The periplasmic binding protein (PBP) CeuE1 is an important component of the Fe(III) uptake system in Campylobacter jejuni, a commensal Gram-negative bacterium in the avian gut, but a common source of food poisoning in humans. CeuE, an integral part of the CeuBCDE ABC transporter of C. jejuni, is responsible for capturing Fe(III)-siderophore complexes in the periplasm for delivery to their respective inner membrane transporter. C. jejuni does not itself synthesize siderophores, but capitalizes on their secretion by other bacteria, such as E. coli. Here we report a combined solution and structural study of a series of synthetic tetradentate analogues of the enterobactin-derived bis(2, 3-dihydroxybenzoyl-L-Ser), to explore the ligand-binding promiscuity of CeuE, both wild type and with mutations of the Fe(III) binding residues H227 and Y288.

Fe(III) complexes of 5-LICAM4−, 6-LICAM4− and 8-LICAM4− were co-crystallized with CeuE and their crystal structures determined. The structural differences can be quantified by calculating the mean planes defined by the six carbon atoms of the two catecholate rings, and measuring their inter-planar angle which is 97°, 111°, 110° and 110° in CFe-4-Lic, CFe-5-Lic, CFe-6-Lic and CFe-8-Lic, respectively. In contrast, the longer and more flexible linkers in Fe-5-Lic, Fe-6-Lic and Fe-8-Lic can adapt to both the geometric requirements of the Fe(III) center and the binding pocket of CeuE. The Kd values of Fe-4-Lic and Fe-6-Lic are similar and lie within three standard deviations of one another. This indicates that the entropic cost incurred upon binding of the ligand with the more flexible 6-atom linker is compensated by its ability to accommodate the preferred octahedral coordination geometry of Fe(III). In addition, the affinities of CeuE for Fe-4-Lic, Fe-5-Lic, Fe-6-Lic and Fe-8-Lic were determined using fluorescence quenching, which yielded dissociation constants of 21 ± 6 nM, < 10 nM, 33 ± 8 nM and 58 ± 8 nM, respectively. The crystal structures of all three complexes show that the siderophore analogues are bound in the Λ-configuration, as previously reported for CFe-4-Lic20, (CeuE)2-[(Fe(MECAM))2]6− 19, FeuA-[Fe(MECAM)]3−, FeuA-[Fe(enterobactin)]3− and FeuA-[Fe(bacillibactin)]32728.

> AMLPISMSDEGDSFLVKDSLGENKIPKNPSKVVILDLGILDTFDALKLNDKVVGVPAKNLPKYLQQFKNKPSVGGVQQVDFEAINALKPDLIIISGRQSKFYDKLKEIAPTLFVGLDNANFLSSFENNVLSVAKLYGLEKEALEKISDIKNEIEKAKSIVDEDKKALIILTNSNKISAFGPQSRFGIIHDVLGINAVDENIKVGTHGKSINSEFILEKNPDYIFVVDRNVILGNKERAQGILDNALVAKTKAAQNKKIIYLDPEYWYLASGNGLESLKTMILEIKNAVK> TQKAPSVQVYFRHPAEKGKENTFHCYAESFHPPKINITLLKNGIPMENVQQSDLSFKKDWTFERLVYAKVIPDGKAEFACKVEHITLPQ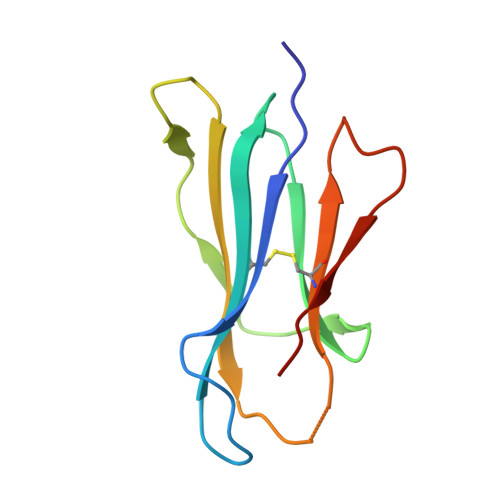PMIYKLDQEY> MA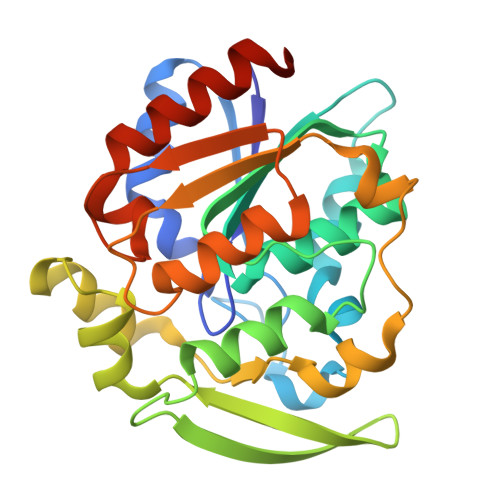FAHFVLIHGICHGAWIWHKLKPLLEALGHKVTALDLAASGVDPRQIEEIGSFDEYSEPLLTFLEALPPGEKVILVGHSLGGLNIAIAADKYCEKIAAAVFVASVLPDTEHCPSYVVDKLMEVFPDWKDTTYFTYTKDGKEITGLKLGFTLLRENLYTLCGPEEYELAKMLTRKSSLFQNILAKRPFFTKEGYGSIKKIYVWTDQDEIFLPEFQLWQIENYKPDKVYKVEGGDHMLQLTKTKEIAEILQEVADTYNLEHHHHHH> PETRPNHTIYINNLNEKIKKDELKKSLHAIFSRFGQILDILVSRSLKMRGQAFVIFKEVSSATNALRSMQGF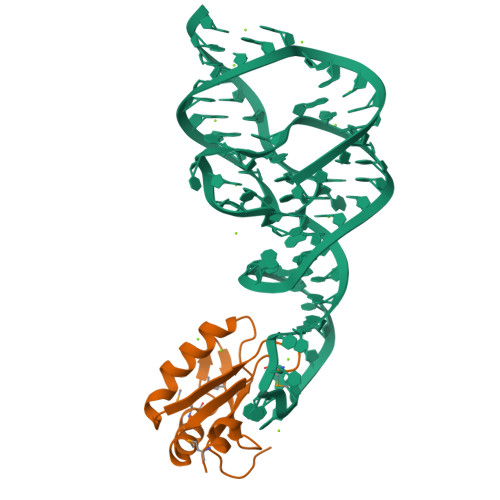PFYDKPMRIQYAKTDSDIIAKMA> LPLNLCFAAIREDDLLLHQLLKRGLDP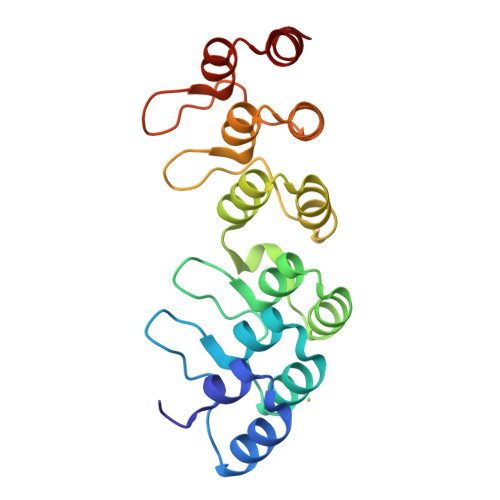NESDNNGRTPLHIAASKGTLNCVLLLLEYHADPNCRDAEGSVPLWEAMVEGHEKVVKVLLEHGSTIDAGDVGHFACTAAEQGNLKLLKEIVLHGGDVTRPRATGTSALHTAVCEENIEMVKYLLEQGADVNKQDMHGWTPRDLAEQQGHEDIKALFRE> SFGSRSDSRGKSSFFS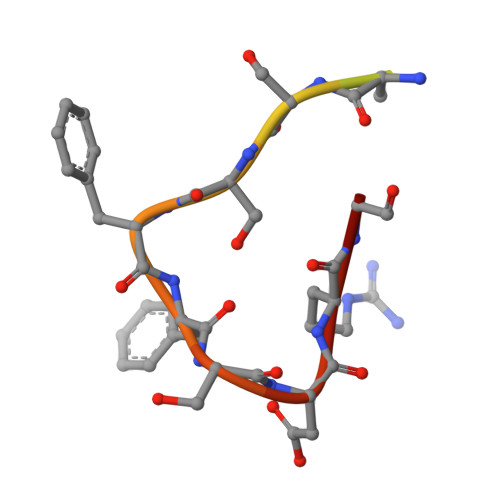DRGS> AFDGT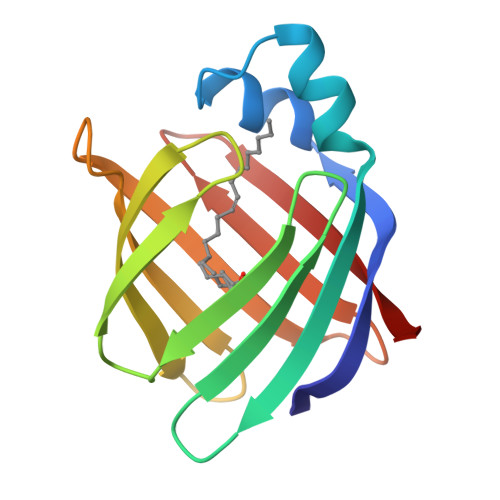WKVDRNENYEKFMEKMGINVVKRKLGAHDNLKLTITQEGNKFTVKESSNFRNIDVVFELGVDFAYSLADGTELTGTWTMEGNKLVGKFKRVDNGKELIAVQEISGNELIQTYTYEGVEAKRIFKKE> MGTITSYAVVFDAGSTGSRVHVYHFDQN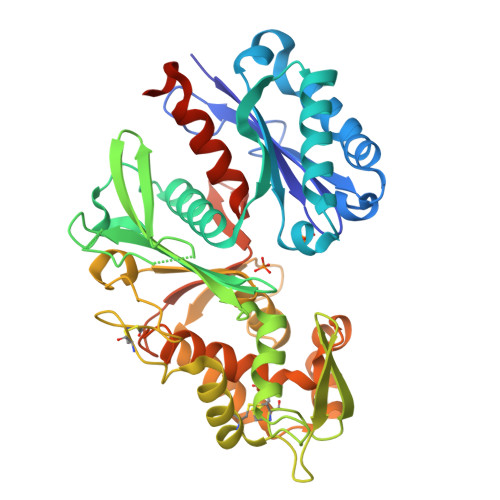LDLLHIGKDVEFYNKIQPGLSAYADNPEQAAKSLIPLLEQAENVVPEDFHSKTPIRLGATAGLRLLDGDASERILQAVRDMLNNKSTFNVQPDAVSIIDGTQEGSYLWVTINYVLGNLGKRFTNTVGVIDLGGGSVQMAYAVSKKTARNAPKVTDGEDPYIKKIVLKGKPYDLYVHSYLHFGREASRAEILKVTHGSASPCILAGFDGIYTYSGEEFKASAPTSGANFDKCKKIIQKALKLDYPCPYQNCTFGGIWNGGGGSGQKKLFAASSFFYLPQDVGMVDPNKSNLKLRPVDLENKAKIVCTLNVEDVKSAYPLLEKFNIVPYACMDLIYQYELLVDGFGLDPLQEITAGEKIEYQEALVDAAWALGNAVEAVLLLPKFERLMYFVVEHHHHHH> MPKTLTEKLNAIKAAGKGIFVPYIMAGDHEKGLDGLAETIHFLEDLGVSAIEVGIPFSDPVADGPVIEEAGLRSLAHGTSTQALVETLKTIETEIPLVIMTYFNPLFQYGVENFVKDLADTAVKGLIIPDLPHEHANF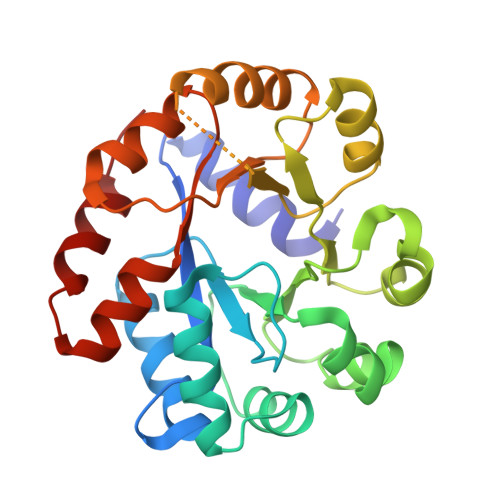VEPFLANTDIALIPLVSLTTGIERQKELIEGAEGFIYAVAINGVTGKSGNYRADLDKHLAQLHQVADIPVLTGFGVSSQADLERFNAVSDGVIVGSKIVKALHQGEPIQDFIRQAVAYQK>GPNMKERIHEYCHRLHLPVMAERWSAMAEYASTHNISYSEFLFRLLEAEIVEKQARSIQTLIKLSKLPYRKTIDTFDFTAQPSVDERRIRELLTLSFIDRKENILFLGPPGIGKTHLAISIGMEAIARGYKTYFITAHDLVNQLRRADQEGKLEKKLRVFVKPTVLIIDEMGYLKLDPNSAHYLFQVIARRYEHAPIILTSNKSFGEWGEIVGDSVLATAMLDRLLHHSIIFNLKGESYRLREKRLQEEKQKDQ[10x]

Using IS21 as a model transposase system, we show how an ATPase regulator uses nucleotide-controlled assembly and DNA deformation to enable structure-based site selectivity, transposase recruitment, and activation and integration. The IstA transposase possess two helix-turn-helix (HTH) DNA-binding domains, a DDE catalytic motif and a β-barrel followed by a flexible carboxy-terminal region21. IstB, similar to the MuB and TnsC helper proteins, is a member of the AAA+ family and a close paralogue of the DnaC/I helicase loader. However, this tetramer state is inactive and requires the regulatory IstB factor to perform transposition.

A 3.2 Å resolution structure of IstB bound to target DNA reveals how specific elements of the N-terminal dimerization and AAA+ ATPase domains facilitate protein oligomerization to engage and bend a 60 bp duplex while maintaining an ATPase-repressed state. In accord with previous low-resolution studies, the cryo-EM structure showed that IstB utilizes its N-terminal domains to form dimers that oligomerize into a clamshell-shaped, two-fold symmetric decamer through ATP-dependent AAA+ domain interactions. That is, the inverted arrangement of two AAA+ domain pentamers, the DNA-binding surfaces of which face one another owing to the molecular two-fold axes of their associated N-terminal domains, sterically prevents the binding of a sixth ATPase subunit to the complex in this configuration. In the IstB decamer, eight out of the ten nucleotide-binding sites adopt a canonical AAA+ ATPase configuration. Close inspection of the EM map showed clear density maps for ATP in all binding pockets. Exceptions were the two terminal monomers where the nucleotide-binding sites are solvent exposed (the outer dimers are also more flexible). The first 65 residues of IstB are composed of 3 small α-helices, which form the dimerization interface of the protein and connect through an elongated helical extension to the AAA+ domain. Close inspection of the complex revealed the presence of numerous positively charged residues that interact with the target DNA, which partially explained the 30-fold increase in duplex affinity observed for the full-length protein compared with the isolated ATPase module (Kd,app of 40 nM versus 1.5 µM, respectively). These amino acids, together with a conserved region of the AAA+ domains known as the initiator-specific motif, form an internal cavity within each IstB dimer that engages DNA primarily through nonspecific contacts to the phosphodiester backbone. The subsequent assembly of IstB dimers into the final decameric state in turn generates a continuous, U-shaped channel that tracks the periodicity of the duplex DNA (about 10.5 bp) and introduces an approximate 180° curve into the target molecule.1,3-benzothiazole-2,5-disulfonic acid | C7 H5 N O6 S3 | 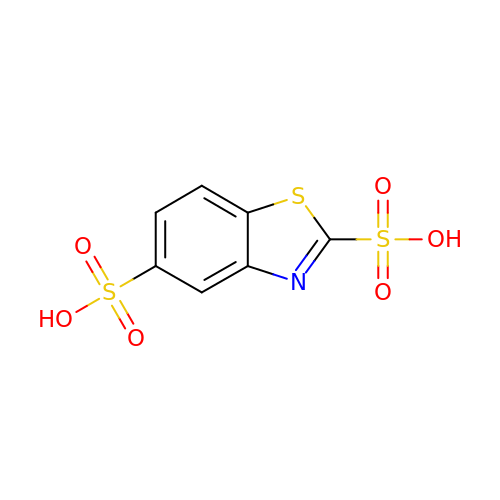LPQVEXUZOUXFTH-UHFFFAOYSA-N>[4x]MKHHHHHHMHHHHHHENLYFQGWQENKSWNAHFTEHKSQGVVVLWNENKQQGFTNNLKRANQAFLPASTFKIPNSLIALDLGVVKDEHQVFKWDGQTRDIATWNRDHNLITA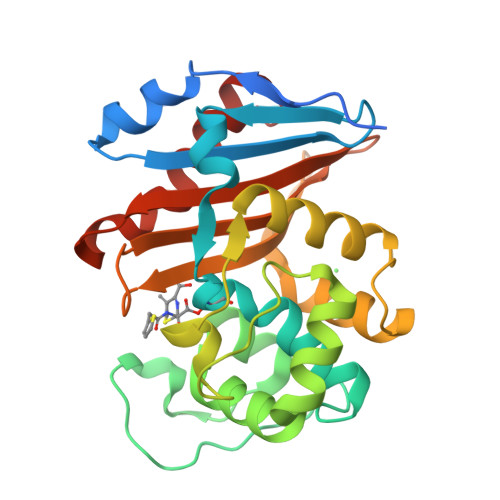MKYSVVPVYQEFARQIGEARMSKMLHAFDYGNEDISGNVDSFWLDGGIRISATEQISFLRKLYHNKLHVSERSQRIVKQAMLTEANGDYIIRAKTGYSTRIEPKIGWWVGWVELDDNVWFFAMNMDMPTSDGLGLRQAITKEVLKQEKIIP>[3x]HHHHHHSGNTIVNGAPAINASLNIAKSETKVYTGEGVDSVYRVPIYYKLKVTNDGSKLTFTYTVTYVNPKTNDLGNISSMRPGYSIYNSGTSTQTMLTLGSDLGKPSGVKNYITDKNGRQVLSYNTSTMTTQGSGYTWGNGAQMNGFFAKKGYGLTSSWTVPITGTDTSFTFTPYAARTDRIGINYFNGGGKVVESST

The pneumococcal serine rich repeat protein (PsrP), present in 60% of strains capable of causing pneumonia in children, has been identified as a key factor for biofilm formation using in vitro and in vivo models. PsrP belongs to the serine rich repeat protein (SRRP) family found in Gram-positive bacteria. SRRPs are attached to the capsular surface via a cell wall anchoring domain and display a long, highly repetitive and glycosylated C-terminal serine rich-repeat (SRR) region. Although the fold topology of the BR domain of PsrP compared to the other BR domains could not be predicted due to very low sequence similarity, the recently determined crystal structure of the KRT10-binding domain of PsrP (BR187–385) revealed a topology distantly related to the CnaA fold.

However, during purification of the heterologously produced BR187–385, higher oligomer states were formed in the final size exclusion chromatography (SEC) step. Interestingly, these isolated oligomer populations were stable in solution but not in steady-state equilibrium with the monomer, as demonstrated using AUC and SEC. Since stable oligomer formation of PsrP could be relevant for pneumococcal biofilm formation, crystallization trials were set up for the isolated BR187–385 dimer in order to obtain a molecular understanding for stable dimer formation. Therefore, a shorter construct was designed by deleting the seven C-terminal residues in BR187–385 that were not built in the previously determined crystal structure due to missing electron density. Well-diffracting crystals were obtained of the isolated irreversibly associated BR187–378 dimer. Analysis of the crystal structure solved by molecular replacement revealed that the residue stretches L202-G315 (region I) and Y316-S377 (region II) are reciprocally exchanged between two separate chains. This reciprocal exchange of entire protein segments is termed 3D-domain swapping and has been first described for diphtheria toxin. A common feature of domain-swapped oligomers is the requirement to pass a high-energy barrier between the non-swapped and swapped states. Thus, it should be noted that the irreversibly associated dimers were only obtained following heterologous production of the isolated BR protein constructs, and that, at this stage, we remain uncertain about their formation in vivo. Moreover, intermolecular β-sheets are also observed between symmetry-related domain-swapped dimers with similar interfaces and hydrogen bond patterns.>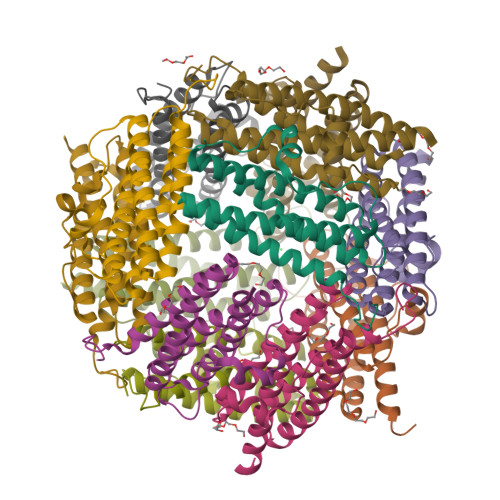[12x]MSATTTLKEQVLTTLKREQANAVVMYLNYKKYHWLTYGPLFRDLHLLFEEQGSEVFAMIDELAERSLMLDGQPVADPADYLKVATVTPSSGQLTVKQMIEEAIANHELIITEMHQDAEIATEAGDIGTADLYTRLVQTHQKHRWFLKEFLAKGDGLVS>[2x]MNDAPPFDLDAYLARIGYTGPRNASLDTLKALHFAHPQAIPFENIDPFLGRPVRLDLAALQDKIVLGGRGGYCFEHNLLFMHALKALGFEVGGLAARVLWGQSEDAITARSHMLLRVELDGRTYIADVGFGGLTLTAPLLLEPGREQKTPHEPFRIVEADDHFRLQAAIGGDWRSLYRFDLQPQYEVDYSVTNYFLSTSPTSHFL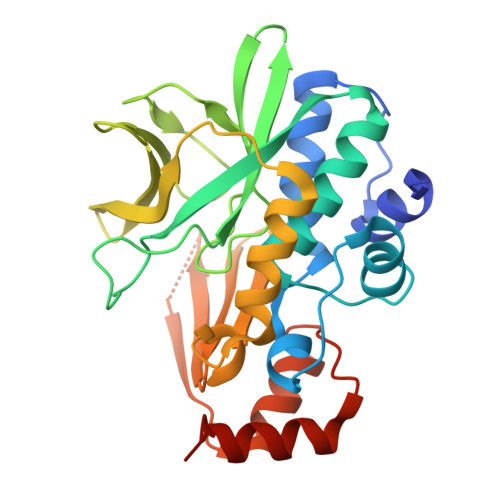SSVIAARAAPDRRYALRGNRLSIHHLGGRTEQTEIATAADLADTLQGLLGIIIPDRTAFEAKVRETKIVETNA> MSGMLDELFSLLNKMFELSDKYRELRKELRKAIESGAPEEELRELLEKMLEIAKKLLELTKELKKLVEDVLKNNPDPVERAKAVLLYAVGVHILYSESSELEVIAERLG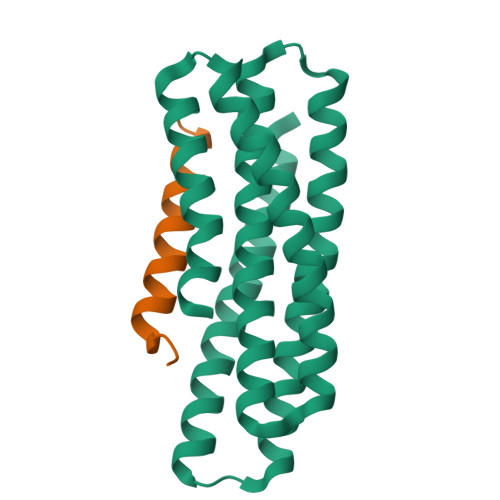FKDIAEKAKEIADKARELKEEVKRKLREIREEVPDPEIRKAAEEAIEMLESNDKRLKEFRKLHSQ;> GFTSDYSKYLDSRRAQDFVQWLMNT>[2x]MRSRRVDVMDVMNR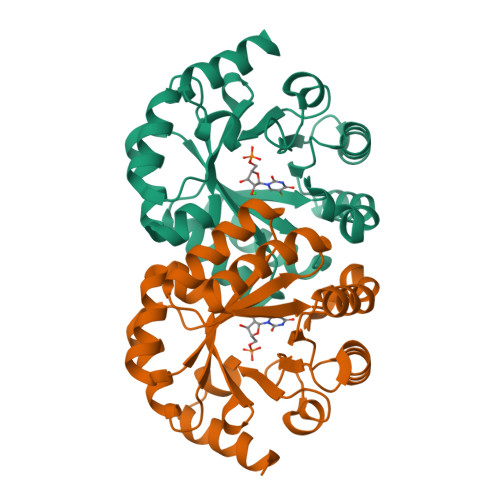LILAMDLMNRDDALRVTGEVREYIDTVKIGYPLVLSEGMDIIAEFRKRFGCRIIAGFKVADIPETNEKICRATFKAGADAIIVHGFPGADSVRACLNVAEEMGREVFLLTEMSHPGAEMFIQGAADEIARMGVDLGVKNYVGPSTRPERLSRLREIIGQDSFLISPGVGAQGGDPGETLRFADAIIVGRSIYLADNPAAAAAGIIESIKDLLNP(2S,3R,4S,5S,6R)-2-[(1S,2S,3R,4S,6R)-3-[(2R,3R,4R,5S,6R)-6-(aminomethyl)-3-azanyl-4,5-bis(oxidanyl)oxan-2-yl]oxy-4,6-bis(azanyl)-2-oxidanyl-cyclohexyl]oxy-6-(hydroxymethyl)oxane-3,4,5-triol | C18 H36 N4 O11 | 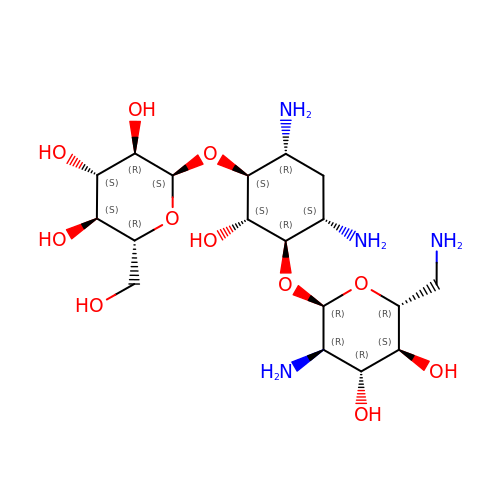MOWMHIINUAQFMU-DNBVWFFRSA-N>GPLGSPLIGEIGPETYSDYMSAGIPLAYIFAETAEERKELSDKLKPIAEAQRGVINFGTIDAKAFGAHAGNLNLKTDKFPAFAIQE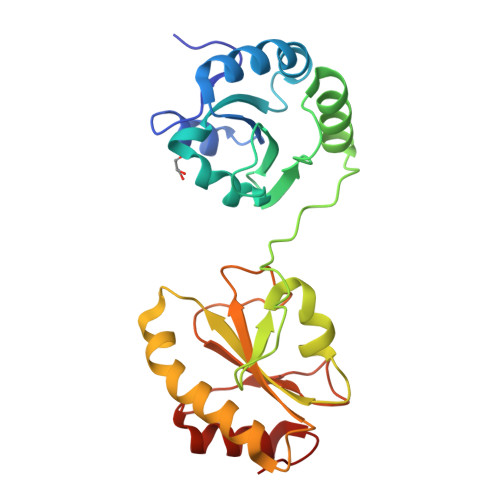VAKNQKFPFDQEKEITFEAIKAFVDDFVAGKIEPSIKSEPIPEKQEGPVTVVVAKNYNEIVLDDTKDVLIEFYAPWCGHCKALAPKYEELGALYAKSEFKDRVVIAKVDATANDVPDEIQGFPTIKLYPAGAKGQPVTYSGSRTVEDLIKFIAENGKYKAA[4x]>GPGGSPYLITGIPKDPKHPLPIRKDIDDWYLEQTSAGSNRIQLTLFVEALTVIQNRPLNDQLSYFRLAGIHGAPWTEWDGVPGGQKDSKGNPTGFCVHNNYTFPTWHRVYVTLYEQVIYEAMLDFIKQNVPQNGKADWENEAKQWRLPYWDFARFARHGHDNTQGDELRLPILVTMPMVKVLVPGQPGKQLSKPNPLYRFQMQTLMGTLERPYAITSQKT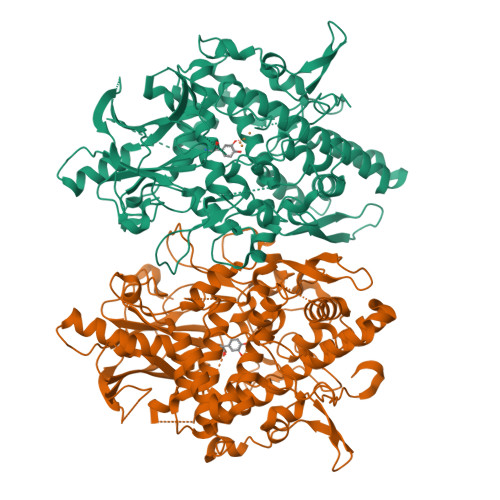EEHGWSFDLPFDKCQSTTKYGLLENYNADVWADGGQNWLRANLALNEHPWYQNLDGWDSVPTLQDMTFRLLTTGGLNWGEFSSTRYDDKKEETQPKNNEQAPKNWMNLEAIHNNVHNWVGGFMFSRPGRHDLKLWGAGHMSSVPVAAYDPIFWLHHCNIDRLTAIWQTVNSGSWFNDDKSKVSKDDDLRPFHRFCEKTRKVVFFRSDDVKDWRSLNYDYAITKDASRIRKEISDLYGQRTKEVYKDFGEEDYILSIRYSRYALGGKPFQINIFFGDVDGKDFYDARSQNFVGSVFNYSGSLEDSNCDKCAQQEQEGVLSVSQLPARLAVHYYKKQNKGEVPTPRYVVVNSQGKAEAEVKVEVALHKTEGTFYDAPARGGSDDYRRVADGKRAEVDDAYRA[2x]>MATVENFNELPAHVWPRNAVRQEDGVVTVAGVPLPDLAEEYGTPLFVVDEDDFRSRCRDMATAFGGPGNVHYASKAFLTKTIARWVDEEGLALDIASINELGIALAAGFPASRITAHGNNKGVEFLRALVQNGVGHVVLDSAQELELLDYVAAGEGKIQDVLIRVKPGIEAHTHEFIATSHEDQKFGFSLASGSAFEAAKAANNAENLNLVGLHCHVGSQVFDAEGFKLAAERVLGLYSQIHSELGVALPELDLGGGYGIAYTAAEEPLNVAEVASDL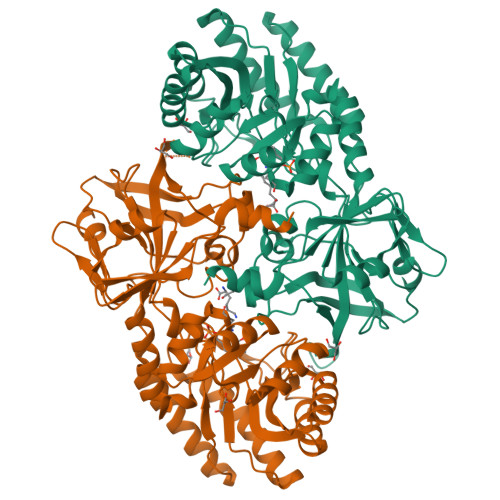LTAVGKMAAELGIDAPTVLVEPGRAIAGPSTVTIYEVGTTKDVHVDDDKTRRYIAVDGGMSDNIRPALYGSEYDARVVSRFAEGDPVSTRIVGSHCESGDILINDEIYPSDITSGDFLALAATGAYCYAMSSRYNAFTRPAVVSVRAGSSRLMLRRETLDDILSLEALEHHHHHH[2x]> PISPIETVPVKLKPGMDGPKVKQWPLTEEKIKALVEICTEMEKEGKISKIGPENPYNTPVFAIKKKDSTKWRKLVDFRELNKRTQDFWEVQLGIPHPAGLKKNKSVTVLDVGDAYFSVPLDEDFRKYTAFTIPSINNETPGIRYQYNVLPQGWKGSPAIFQSSMTKILEPFKKQNPDIVICQYMDDLYVGSDLEIGQHRTKIEELRQHLLRWGLTTPDKKHQKEPPFLWMGYELHPDKWTVQPIVLPEKDSWTVNDIQKLVGKLNWASQIYPGIKVRQLCKLLRGTKALTEVIPLTEEAELELAENREILKEPVHGVYYDPSKDLIAEIQKQGQGQWTYQIYQEPFKNLKTGKYARMRGAHTNDVKQLTEAVQKITTESIVIWGKTPKFKLPIQKETWETWWTEYWQATWIPEWEFVNTPPLVKLWYQLEKEPIVGAETFYVDGAANRETKLGKAGYVTNKGRQKVVPLTNTTNQKTELQAIYLALQDSGLEVNIVTDSQYALGIIQAQPDKSESELVNQIIEQLIKKEKVYLAWVPAHKGIGGNEQVDKLVSAGIR;> PISPIETVPVKLKPGMDGPKVKQWPLTEEKIKALVEICTEMEKEGKISKIGPENPYNTPVFAIKKKDSTKWRKLVDFRELNKRTQDFWEVQLGIPHPAGLKKNKSVTVLDVGDAYFSVPLDEDFRKYTAFTIPSINNETPGIRYQYNVLPQGWKGSPAIFQSSMTKILEPFKKQNPDIVICQYMDDLYVGSDLEIGQHRTKIEELRQHLLRWGLTTPDKKHQKEPPFLWMGYELHPDKWTVQPIVLPEKDSWTVNDIQKLVGKLNWASQIYPGIKVRQLCKLLRGTKALTEVIP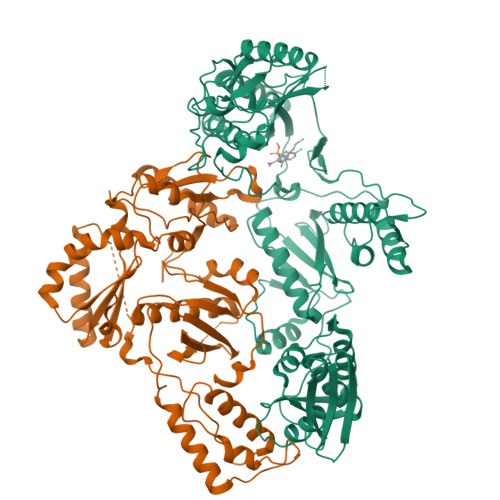LTEEAELELAENREILKEPVHGVYYDPSKDLIAEIQKQGQGQWTYQIYQEPFKNLKTGKYARMRGAHTNDVKQLTEAVQKITTESIVIWGKTPKFKLPIQKETWETWWTEYWQATWIPEWEFVNTPPLVKLWYQLEKEPIVGAETF> VEEVIEMQGLSLDPTSHRVMAGEEPLEMGPTEFKLLHFFMTHPERVYSREQLLNH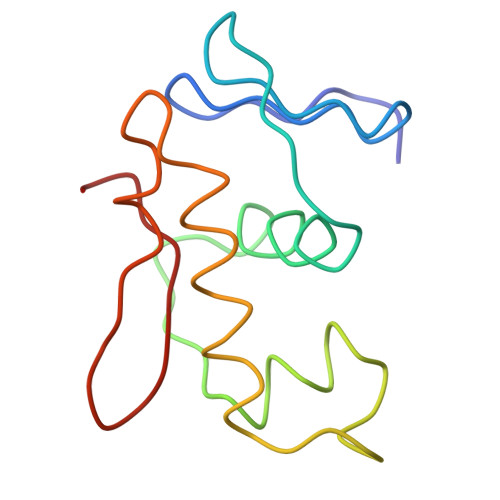VWGTNVYVEDRTVDVHIRRLRKALEPGGHDRMVQTVRGTGYRFSTRF>[4x]SLVELGKMILQETGKNPAKSYGAYGCNCGVLGRGKPKDATDRCCYVHKCCYK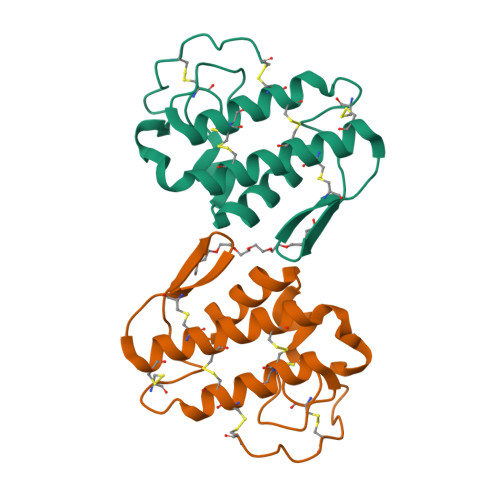KLTNCDPKKDRYSYDWKNKTIVCGEENPCLKQLCECDKAVAICLRENKGTYNKKRDVYLKPFCDKGRDC>AGIHHHHHHSSEPSCRFAHQYTQEQVLQNPSKFINDVLFWEGKFHQNNISYNSGNGMSYDGTNIDWVTGEGTVKHPFSAASKESLQVMLYAHAIAGSADAARFLSPNNPSAAPGIAASIMDTKLQTYLRFNETYPGFGGFLPWFTSSSQDLTPTWDWNNRVPGLDNGELLWAVYAFIQAAENTSNKSFIDLAKKWQTWMDYTKTTAAHIFYQGEGKVCAVTDIKNQSLPVYHPEQTYACEGTSYLNDPYEGELFTWWLQFFGGL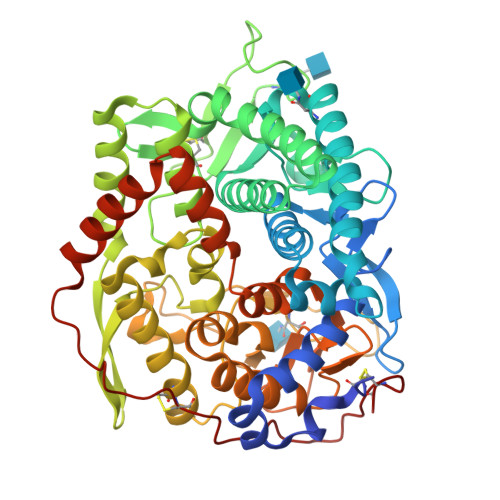SDADIEALWEYKRPQLVSVDYHIGNVGPITVQKGYWFSSHETWKVLEMPYYDIDIIRRVFQNAERARTCNSVVTQVPGMFASINNVTDPATGDVVGYISNAGIPSIANQTIQELDVITPYSVFPTVLFDKGVGMAWWRNMAIGKKMQNIYGSTESTRRDGTGVSALLTWDSKVSTVNAILGGVSGLVSQKMKAENIYNTFVERIEAEYSRVFKNLKGEHVPFCLPQETVPDTGLVDFTTCN[2x]> AHRPARVDIAMPTTSSPTAGETWLILGTDSRATVPGDQNRYGTTQEVEGSRADVIALVRPSQEGVTIINLPRDLTINSKGMELDRLATTYVPGPQNTVNALCTGLGIPTTHLVTIDMAQFATIIDSLGGIEVDVPEPVRDAYTGLNLSSAGRHRLSGID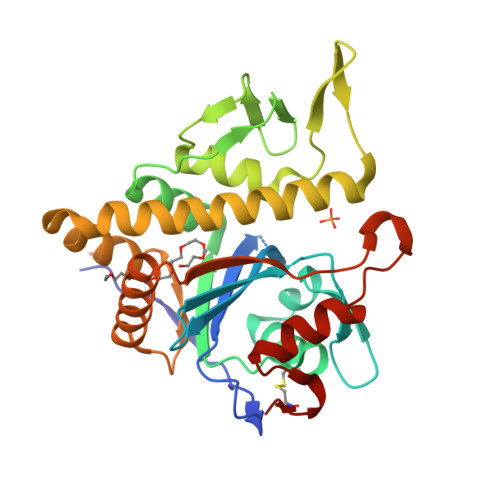ALALVRSRHPEILRDGRWVTMSQADGAQRRSQSTATVMQAVLSAIGQKASNPVSLHQLAHTVAGNITLDSGTGLSDLAALGRSASKARRAGATTIIDLPTGPRDESIIVSPNQESRDLLARYGYSPKTCRPAGA>[2x]MHHHHHHGSGSENLYFQGMETTDTKREEQEIEEKKAQEESKIEDVDKILNDILSISSECIQPDELRVKLLLKRKLICYDGFEPSGRMHIAQGLLKSIIVNKLTSNGCT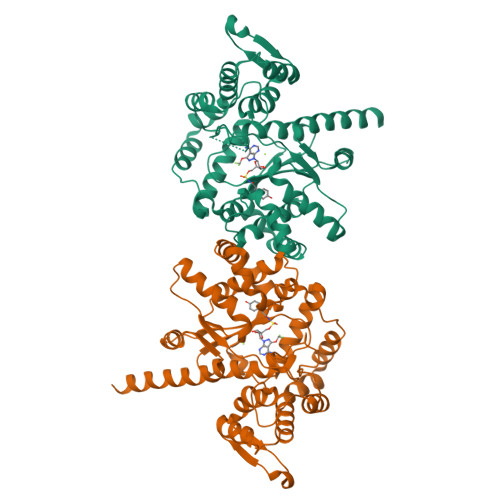FIFWIADWFAHLNNKMSGDLKKIKKVGSYFIEVWKSCGMNMENVQFLWASEEINKKPNEYWSLVLDISRSFNINRMKRCLKIMGRSEGEENYCSQILYPCMQCADIFFLNVDICQLGIDQRKVNMLAREYCDIKKIKKKPVILSHGMLPGLLEGQEKMSKSDENSAIFMDDSESDVNRKIKKAYCPPNVIENNPIYAYAKSIIFPSYNEFNLVRKEKNGGDKTYYTLQELEHDYVNGFIHPLDLKDNVAMYINKLLQPVRDHFQNNIEAKNLLNEIKKYKVTK> MSIIAINENGFLDKIKGRNPLFTCVISSIETTLSIPISGVHRDVIKYTPSADVELVFYGKSLTLKTPPI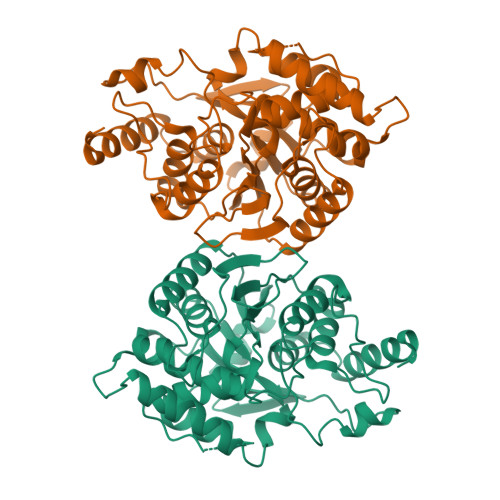DATGSPTPATITRACVELKNIKNLHIDAGAFVKPKIPFIEIDEKPTGRIEEGKAMNNSKELYMKGYLLGKNLDAELLIVGESVPGGTTTALGVLLGLGYDAEGKVSSGSINNPHELKIKVVREGLKKAGINEKSSVFDVLNAVGDKMMPVVAGLAISFAERNKPVILAGGTQMSAVLAVIKEINKKVLDKNLIAIGTTEFVLNDKKGDLKGIVEQIGNVPVLASKFYFEKAKIEGLKNYCKGSVKEGVGAGGIAVYSIVNDLEPTKIREFIENKFYEWYKE>[2x]LPQTVRIGTDTTYAPFS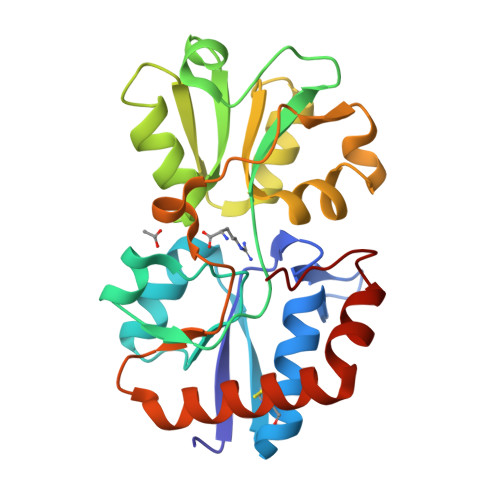SKDAKGEFIGFDIDLGNEMCKRMQVKCTWVASDFDALIPSLKAKKIDAIISALSITDKRQQEIAFSDKLYAADSRLIAAKGSPIQPTLESLKGKHVGVLQGSTQEAYANDNWRTKGVDVVAYANQDLIYSDLTAGRLDAALQDEVAASEGFLKQPAGKEYAFAGPSVKDKKYFGDGTGVGLRKDDTELKAAFDKALTELRQDGTYDKMAKKYFDFNVYGD> MPQLPEVETIRRTL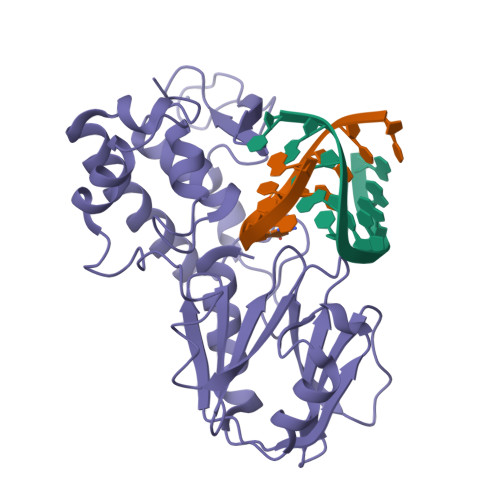LPLIVGKTIEDVRIFWPNIIRHPRDSEAFAARMIGQTVRGLERRGKFLKFLLDRDALISHLRMEGRYAVASALEPLEPHTHVVFCFTDGSELRYRDVRKFGTMHVYAKEEADRRPPLAELGPEPLSPAFSPAVLAERAVKTKRSVKALLLDCTVVAGFGNIYVDESLFRAGILPGRPAASLSSKEIERLHEEMVATIGEAVMKGGSTVRTYVNTQGEAGTFQHHLYVYGRQGNPCKRCGTPIEKTVVAGRGTHYCPRCQR>[2x]AGHMTSMRIPVIRSPLEIRDTERKGRGVFALEPIPAQTCIEISPVLMFSKEEYEQHGQYT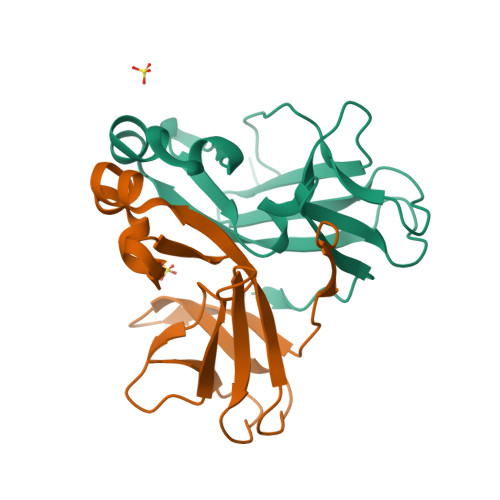VLNEYTYVWSEGKQGLALGLGSMFNHDRHPNVYWKKDNRNNYISYYTLREIKTNEELCISYGDHLWFEDEASSASRISPNEENEDFPLQNISLLETMYPYDVPDYAAPG> TMAASQTSQTVASHVPFADLCSTLERIQKSKGRAEKIRHFREFLDSWRKFHDALHKNHKDVTDSFYPAMRLILPQLERERMAYGIKETMLAKLYIELLNLPRDGKDALKLLNYRTPTGTHGDAGDFAMIAYFVLKPRCLQKGSLTIQQVNDLLDSIASNNSAKRKDLIKKSLLQLITQSSALEQKWLIRMIIKDLKLGVSQQTIFSVFHNDAAELHNVTTDLEKVCRQLHDPSVGLSDISITLFSAFKPMLAAIADIEHIEKDMKHQSFYIETKLDGERMQMHKDGDVYKYFSRNGYNYTDQFGASPTEGSLTPFIHNAFKADIQICILDGEMMAYNPNTQTFMQKGTKFDIKRMVEDSDLQTCYCVFDVLMVNNKKLGHETLRKRYEILSSIFTPIPGRIEIVQKTQAHTKNEVIDALNEAIDKREEGIMVKQPLSIYKPDKRGEGWLKIKPEYVSGLMDELDILIVGGYWGKGSRGGMMSHFLCAVAEKPPPGEKPSVFHTLSRVGSGCTMKELYDLGLKLAKYWKPFHRKAPPSSILCGTEKPEVYIEPCNSVIVQIKAAEIVPSDMYKTGCTLRFPRIEKIRDDKEWHECMTLDDLEQLRGKASGK;> 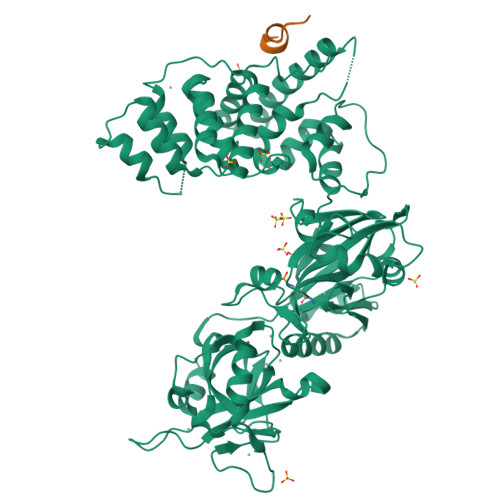DVPQWEVFFKR> KPEPTDEEWELIKTVTEAHVATNAQGSHWKQKRKFLPEDIGQAPIVNAPEGGKVDLEAFSHFTKIITPAITRVVDFAKKLPMFCELPCEDQIILLKGCCMEIMSLRAAVRYDPESETLTLNGEMAVTRGQLKNGGLGVVSDAIFDLGMSLSSFNLDDTEVALLQAVLLMSSDRPGLACVERIEKYQDSFLLAFEHYINYRKHHVTHFWPKLLMKVTDLRMIGACHASW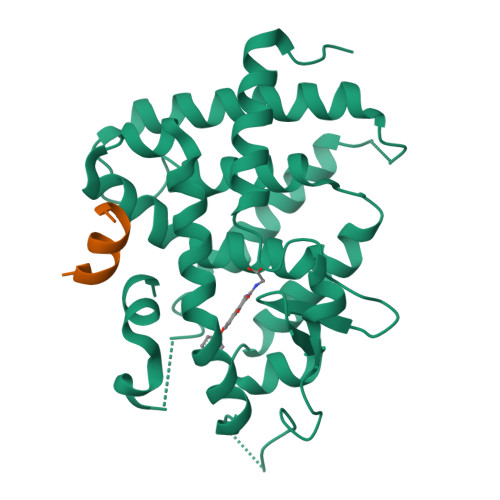FLHMKVECPTELFPPLFLEVFE;> ENALLRYLLDK>[2x]GHMDATDDIR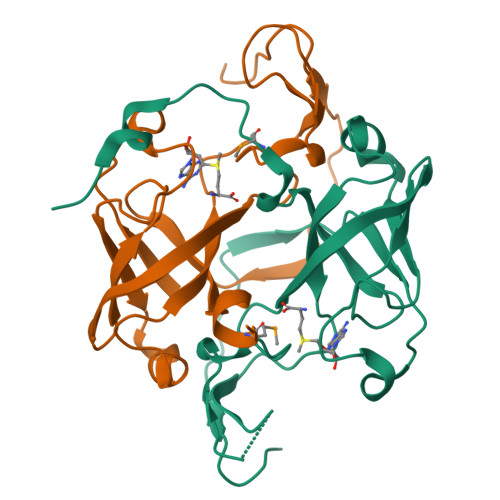AGELASDWSGSPDAGVVFIGRIHTPWNRLKECPRHGRADGPVCRIEVFETWLPALAGIDDGTLLEVFYWLHRSRRDLLLQCPRNDGDARGTFSIRSPLRPNPIGTSIARVDRRDGANLFIRGLDCLDGTPLVDLKPDRAEFMPLAPPKPGDFQVGEPRR>GMSLIPEIDAFLGCPTPDAWIEAALADQETLLIDHKNCEFKAASTALSLIAKYNTHLDLINMMSRLAREELVHHEQVLRLMKRRGVPLRPVSAGRYASGLRRLVRAHEPVKLVDTLVVGAFIEARSCERFAALVPHLDEELGRFYHGLLKSEARHYQGYLKLAHNYGDEADIARCVELVRAAEMELIQSPDQEL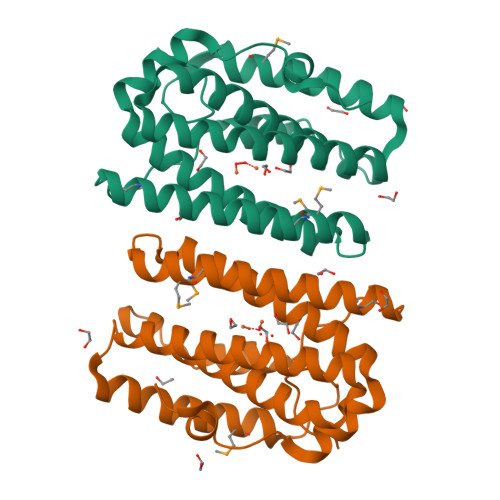RFHSGIPQALAA[2x]(R)-1-(6-(benzylamino)pyrimidin-4-yl)-3-(((6-((4,4-dimethylpiperidin-1-yl)methyl)naphthalen-1-yl)amino)methyl)piperidin-3-ol | C35 H44 N6 O | 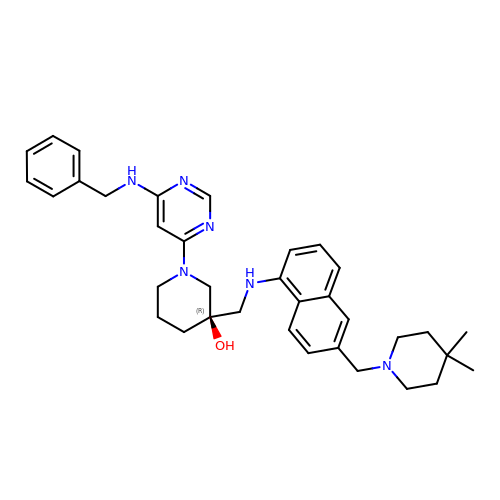JOOQNDNGGGWANB-PGUFJCEWSA-N> MIKSYAAKEAGGELEVYEYDPGELRPQDVEVQVDYCGICHSDLSMIDNEWGFSQYPLVAGHEVIGRVVALGSAAQDKGLQVGQRVGIGWTARSCGHCDACISGNQINCEQGAVPTIMNRGGFAEKLRADWQWVIPLPENIDIESAGPLLCGGITVFKPLLMHHITATSRVGVIGIGGLGHIAIKLLHAMGCEVTAFSSNPAKEQEVLAMGADKVVNSRDPQALKALAGQFDLIINTVNVSLDWQPYFEALTYGGNFHTVGAVLTPLSVPAFTLIAGDRSVSGS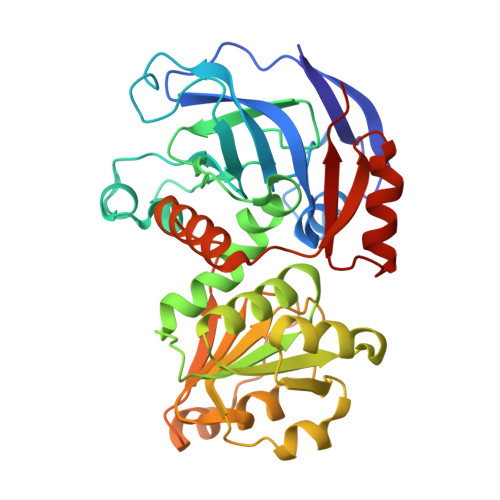ATGTPYELRKLMRFAARSKVAPTTELFPMSKINDAIQHVRDGKARYRVVLKADY4-(6-azanyl-2-chloranyl-purin-9-yl)-~{N}-(4-methyl-1,3-thiazol-2-yl)cyclohexane-1-carboxamide 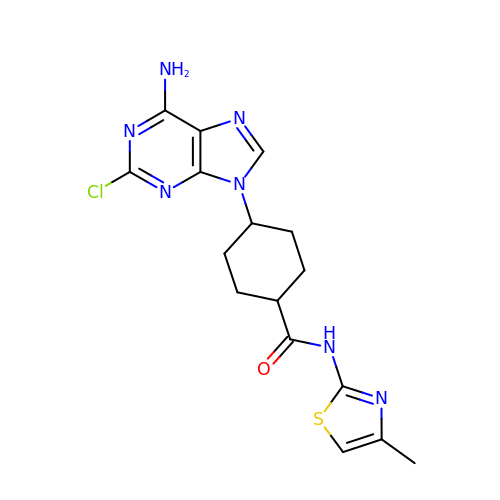| C16 H18 Cl N7 O S | JIOZKGZDCQTDDN-AOOOYVTPSA-N>[2x]GSKRVVTLYQGATDVAVSLGVKPVGAVESWTQKPKFEYIKNDLKDTKIVGQEPAPNLEEISKLKPDLIVASKVRNEKVYDQLSKIAPTVSTDTVFKFKDTTKLMGKALGKEKEAEDLLKKYDDKVAAFQKDAKAKYKDAWPLKASVVNFRADHTRIYAGGYAGEILNDLGFKRNKDLQKQVDNGKDIIQLTSKESIPLMNADHIFVVKSDPNAKDAALVKKTESEWTSSKEWKN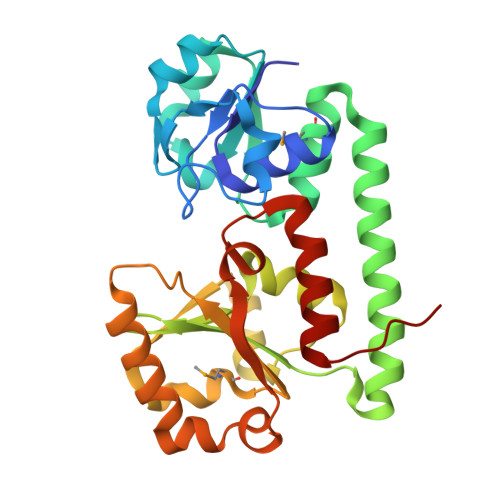LDAVKNNQVSDDLDEITWNLAGGYKSSLKLIDDLYEKLNIEKQSK> GQQVCPNYVMLRSSVTTKVVRNVVEYQIRTGGFFSCLAMLRPLQYAKRERLLGQRNLERISTRDILQTRDLHSLCMPTPDAPMSNHQASTMRELICSYFKVDHADGLKYIPMDERYSPSSLARLFTMGMAGLHITTEPSYKRVPIMHLAADLDCMTLALPYMITLDGDTVVPVAPTLSAEQLLDDGL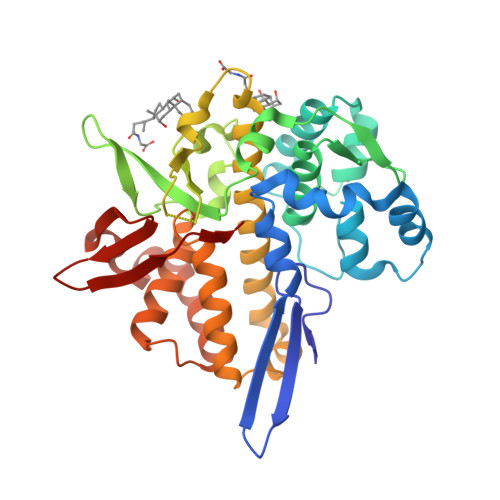KGLACMDISYGCEVDANSRPAGDQSMDSSRCINELYCEETAEAICVLKTCLVLNCMQFKLEMDDLAHNAAELDKIQMMIPFSERVFRMASSFATIDAQCFRFCVMMKDKNLKIDMRETTRLWTRSASDDSVATSSLSISLDRGRWVAADASDARLLVFPIRV1-acetyl-N-(5-methylpyridin-2-yl)piperidine-4-carboxamide | C14 H19 N3 O2 | 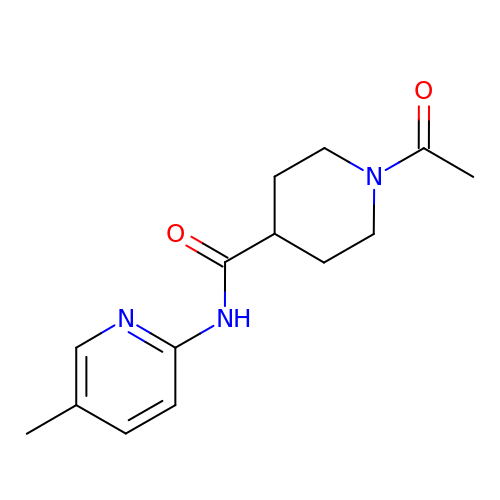LDNVJBRMIHEEJK-UHFFFAOYSA-N> NGPLSCGQR;> VVGGLVALRGAHPYIAALYWGHSFCAGSLIAPCWVLTAAHCLQDRPAPEDLTVVLGQERRNHSCEPCQTLAVRSYRLHEAFSPVSYQHDLALLRLQEDADGSCALLSPYVQPVCLPSGAARPSETTLCQVAGWGHQFEGAEEYASFLQEAQVPFLSLERCSAPDVHGSSILPGMLCAGFLEGGTDACQGDSGGPLVCEDQAAERRLTLQ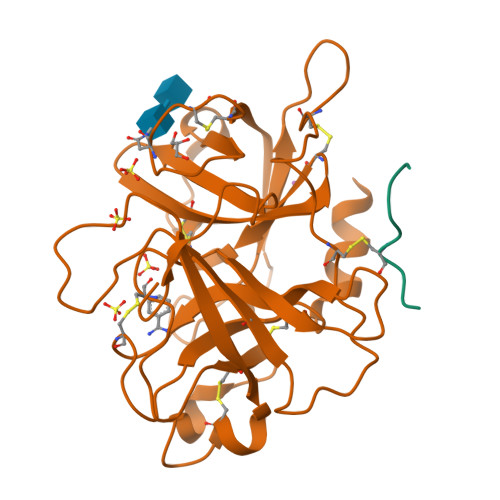GIISWGSGCGDRNKPGVYTDVAYYLAWIREHTVS>[3x]GHMVRSSSRTPSDKPVAHVVANPQAEGQLQWLNRRANALLANGVELRDNQLVVPSEGLYLIYSQVLFKGQ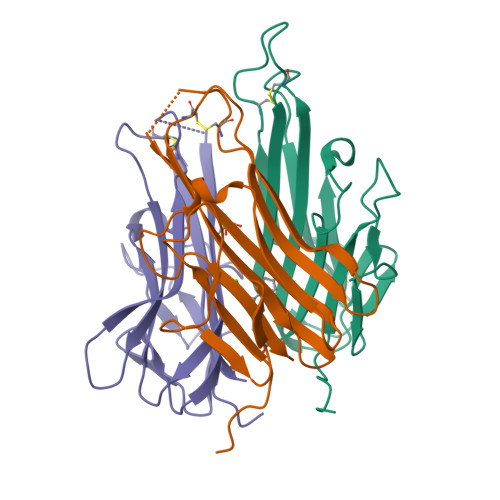GCPSTHVLLTHTISRIAVSYQTKVNLLSAIKSPCQRETPEGAEAKPWYEPIYLGGVFQLEKGDRLSAEINRPDYLDFAESGQVYFGIIAL> MYLTLQEW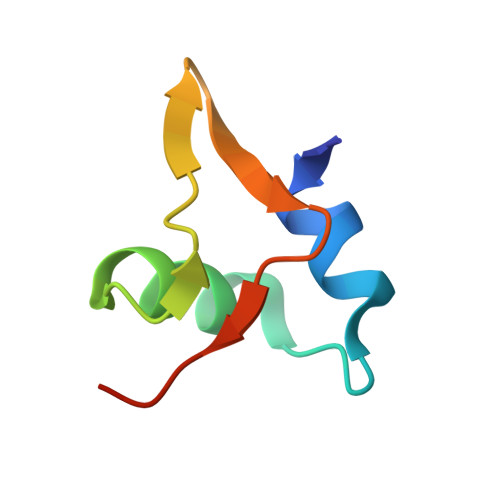NARQRRPRSLETVRRWVRESRIFPPPVKDGREYLFHESAVKVDLNRP> MTNPSPHFFKTFEWPSKAAGLELQNEIEQFYYREAQLLDHRAYEAWFALLDKDIHYFMPLRTNRMIREGELEYSGDQDLAHFDETHETMYGRIRKVTSDVGWAENPPSRTRHLVSNVIVKETATPDTFEVNSAFILYRNRLER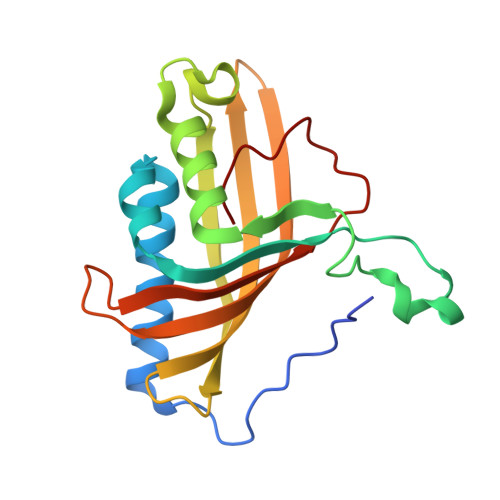QVDIFAGERRDVLRRADNNLGFSIAKRTILLDASTLLSNNLSMFF> MAHHHHHHAELAALEKASNGRLGIAVLDTSNGTRIAHHARERFPLCGTYAVVAAAAIL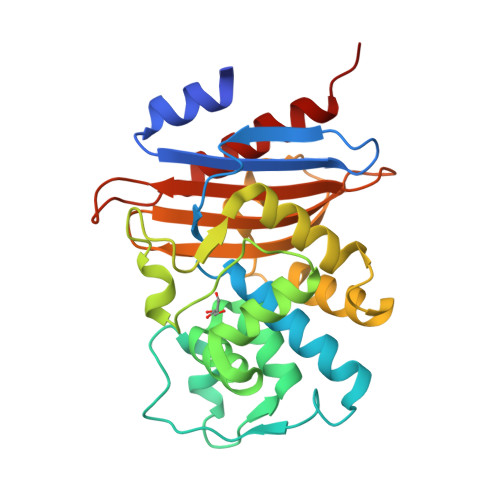ARGSLDASLLPRRILYRRYEVVAGSPVTESHVDTGMTIAQLCAAMLQSGDKGAGNLLMRVLGGPQAVTSFAHESGDTVFRLDRWEPELNLAAPGDERDTSTPVAMVDLLQQLLLGDTLREPQRAQLTEWMTGGARGATAIAAGVPPGWRVADKAGTGGYGTTTDVAVLWPPSRAPIVLAVSFTQPRADAAARADVVASAARIATGALTATA(2~{S})-2-chloranyl-3-(1~{H}-imidazol-5-yl)propanoic acid | C6 H7 Cl N2 O2 | 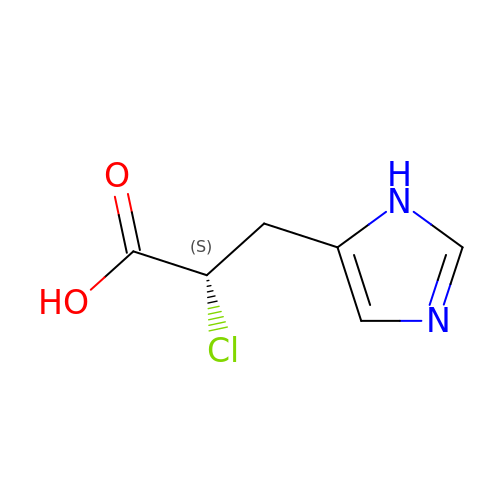JZLQYMHAXPPICX-YFKPBYRVSA-N>MDEESDLKDHRDKWNKYYGVSPDQLSKDLFDKVSPEQIKNSPYQSVGRLNVQGEAVATGVFIGKNTVVTNHHIAKEAKNNPSKIIFSPGRHADESNTGTVLPHGTFEASEIIDAPFGTGVDISVIIFKPNAEGKSIGDVIKAADLGNSNSLKKGDTANLIGYPYDFDSKNMYRSQVEFQSTDFGLKYYGYTVPGNSGSGIFNSEGKF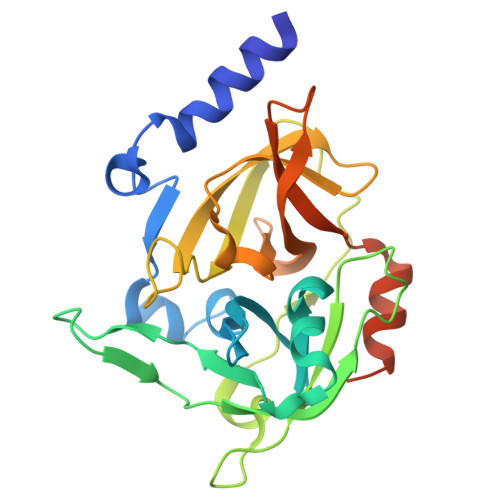VGLHIGKAKHINSQNEINYAVSFNDFLIRDLKQLIKGGENLYFQSHHHHHH[3x]>[2x]GLEAVRKRPGMYIGSTSERGLHHLVWEIVDNSIDEALAGYANQIEVVIEKDNWIKVTDNGRGIPVDIQEKMGRPAVEVILTSSVVNALSQDLEVYVHRNETIYHQAY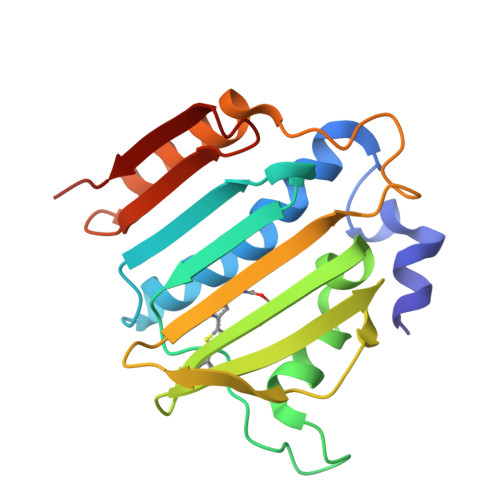KKGVPQFDLKEVGTTDKTGTVIRFKADGEIFTETTVYNYETLQQRIRELAFLNKGIQITLRDERDEENVREDSYHYE> HSQGT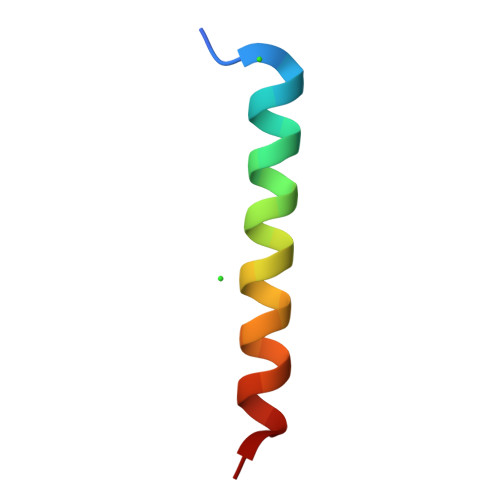FTSDYSKYLDSRRAQDFVQWLMNT>RPMDNEAVQFGMSMGIGWNLGNQMDAHYDGCSYETGWGNKAATQQTFNGLAKAGFRSVRIPVTWMGHIGNAPTYAIERGWLDRVDELVHMAHKAGLIVIINIHHDGFGAADTPSKGSHWLDLPAAVASEERNQLIKQELTMIWLQIGKRFANDGEWLVFETLNAIQDGDWGNGNNRRDGGAQYRVLNEWNQVCVDAIRAAGGKNETRYIGVPGYVCNPDLTVENLVLPEDVVPNRLMVAVHSYDPWDYAGSAKYNEWGHTGKDVVPGVGEEAYVGMLNRLFNMYIRRGVPVYFGEFGAVRRASKADEEFRLYYFRYICKAMRDRRISALYWDNGNSKAGNDGFGVIDHATGRFIGNGEQAVRAMIDSWE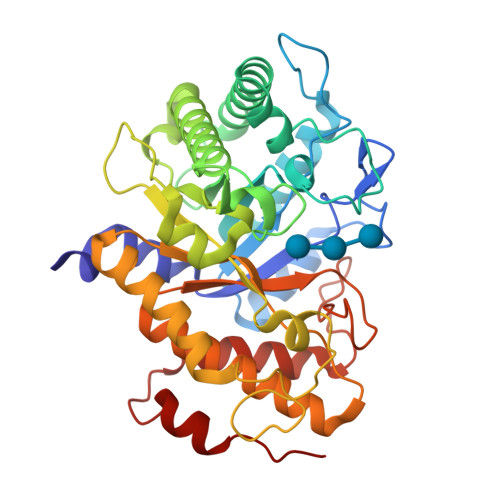NNDPNYTLQSIYDSAPESSR[2x]>[2x]MIIPALNLIGGTVVRVVRLHQGDYARQRDYGNDPLPRLQDYAAQGAGVLHLVDLTGAKDPAKRQIPLIKTLVAGVNVPVQVGGGVRTEEDVAALLKAGVARVVIGSTAVKSPDVVKGWFERFGAQALVLALDVRIDEHGTKQVAVSGWQENSGVSLEQLVETYLPVGLKHVLCTDISRDGTLAGSNVSLYEEVCARYPQIAFQSSGGIGDID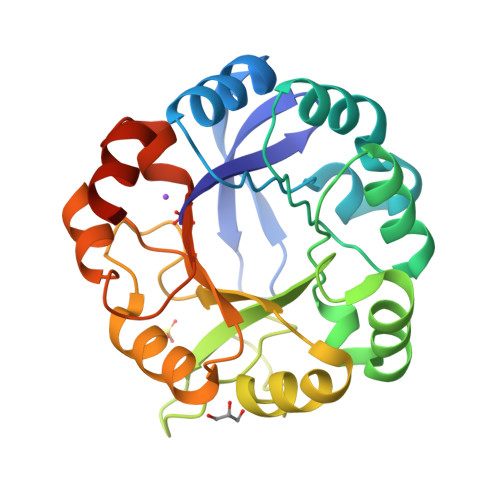DIAALRGTGVRGVIVGRALLEGKFTVKEAIQCWQNVKGHHHHHH> SFTSPAVKRLLGWKGGGSQGDEEEKWAEKAVDALVKKLKKKKGAMEELEKALSSPGQPSKCVTIPRSLDGRLQVSHRKGLPHVIYCRVWRWPDLQSHHELK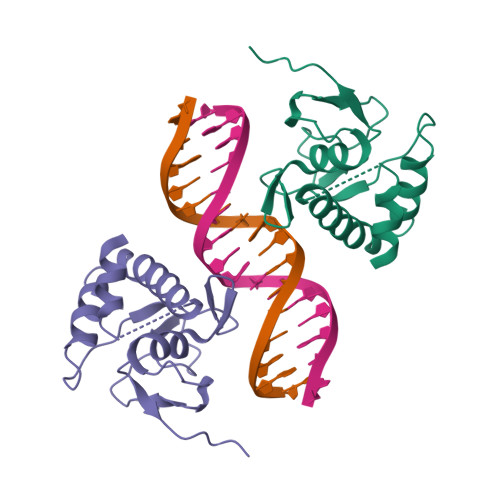PLDICEFPFGSKQKEVCINPYHYKRVESPVLPP>[8x]MVHYKLTYFAGRGLAEPIRQIFALAGQKYEDVRYTFQEWPKHKDEMPFGQIPVLEEDGKQLAQSFAIARYLSRKFG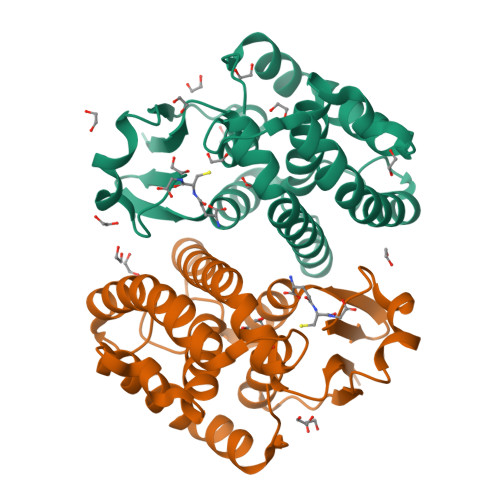FAGKTPFEEALVDSVADQYKDYINEIRPYLRVVAGVDQGDPEKLFKELLLPAREKFFGFMKKFLEKSKSGYLVGDSVTYADLCLAEHTSGIAAKFPSIYDGFPEIKAHAEKVRSIPALKKWIETRPETKF>DYESPIVNVVEACAPAVVKIDVVKTVKTSFFDPYFEQFFKKWFGELPPGFERQVASLGSGFIFDPEGYILTNYHVVGGADNITVTMLDGSKYDAEYIGGDEELDIAVIKIKASDKKFPYLEFGDSDKVKIGEWAIAIGNPLGFQHTVTVGVVSATNRRIPKPDGSGYYVGLIQ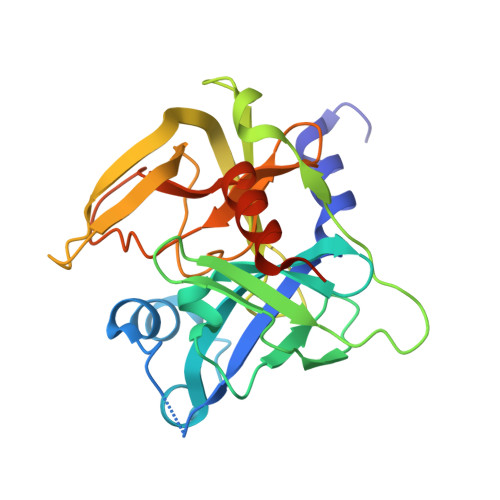TDAAINPGNSGGPLLNIHGEVIGINTAIVNPQEAVNLGFAIPINTVKKFLDTILTQKKVEKAYLGV[2x]>[3x]GSHMSSPVNEEENSQRISTLHHQTMPSDLTQDEFTQLSQSIAEFHTYQLGNGRCSSLLAQRIHAPPETVWSVVRRFDRPQIYKHFIKSCNVSEDFEMRVGCTRD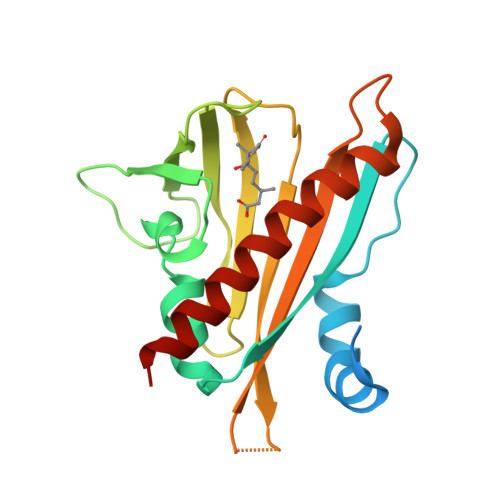VNVISGLPANTSRERLDLLDDDRRVTGFSITGGEHRLRNYKSVTTVHRFEKEEEEERIWTVVLESYVVDVPEGNSEEDTRLFADTVIRLNLQKLASITEAMNRN> GYSDRVRSITLGNSTITTQECANVVVGYGEWPEYLSDNEATAEDQPTQPDVATCRFYTLDSVQWENGSPGWWWKFPDALRDMGLFGQNMYYHYLGR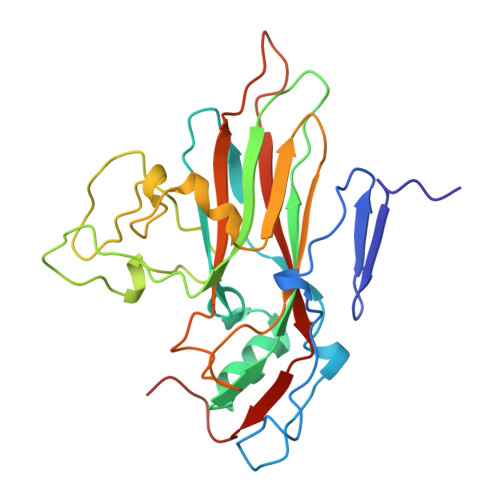AGYTIHVQCNASKFHQGCILVVCVPEAEMGSAQTSGVVNYEHISKGEIASRFTTTTTAEDHGVQAAVWNAGMGVGVGNLTIFPHQWINLRTNNSATIVMPYVNSVPMDNMYRHHNFTLMIIPFVPLDFSAGASTYVPITVTVAPMCAEYNGLRLAGHQ> GPETGNKYIEKRAIDLSRERDPNFFDNADIPVPECFWFMFKNNVRQDAGTCYSSWKMD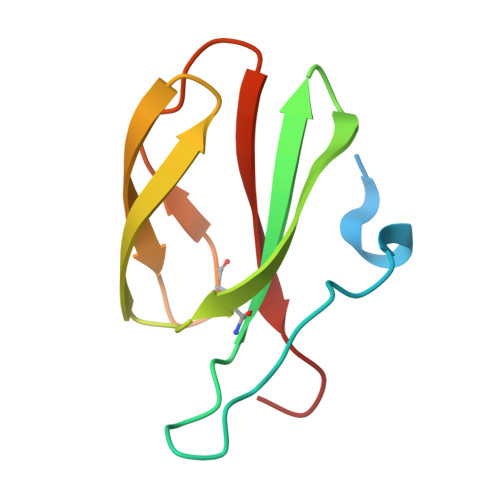KKVGPNWVHIKSDDNCNLSGDFPPGWIVLGKKRPGF> MAQLALALDTVTRYLRLKAPFAAFRPFQSGSFRSTTPVPSFSAVYGLLLNLAGIEQRQEVEGKVTLIKPKAELPKLAIAIGQVKPSSTSLINQQLHNYPVGNSGKEFASRTFGSKYWIAPVRREVLVNLDLIIGLQSPVEFWQKLDQGLKGETVINRYGLPFAGDNNFLFDEIYPIEKPDLASWYCPLEPDTRPNQGACRLTLWIDRENNTQTTIKVFSPSDFRLEPPAKAWQQLPG;>[7x]MSNLNLFATILTYPAPASNYRGESEENRSVIQKILKDGQKYAIISPESMRN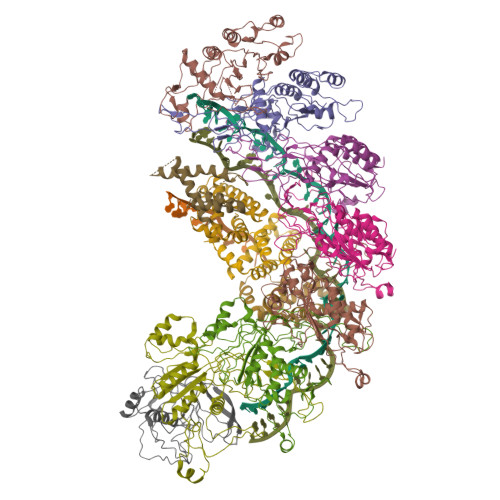ALREMLIELGQPNNRTRLHSEDQLAVEFKEYPNPDKFADDFLFGYMVAQTNDAKEMKKLNRPAKRDSIFRCNMAVAVNPYKYDTVFYQSPLNAGDSAWKNSTSSALLHREVTHTAFQYPFALAGKDCAAKPEWVKALLQAIAELNGVAGGHARAYYEFAPRSVVARLTPKLVAGYQTYGFDAEGNWLELSRLTATDSDNLDLPANEFWLGGELVRKMDQEQKAQLEAMGAHLYANPEKLFADLADSFLGV;>MTVATTKTREYAEIVYKIAQGFVLSKLSSKHDLQWSKCKGNPKLEREYNDKKEKVVNEAFLAIRSRTEKQAFIDYFVSTLYPHVRQDEFVDFAQKLFQDTDEIRSLTLLALSSQYPIKRQGETE[4x]> SSQIRQNYSTEVEAAVNRLVNLYLRASYTYLSLGFYFDRDDVALEGVCHFFCELACEKCEGACRLLKMQNQRGGRALFQDLQKP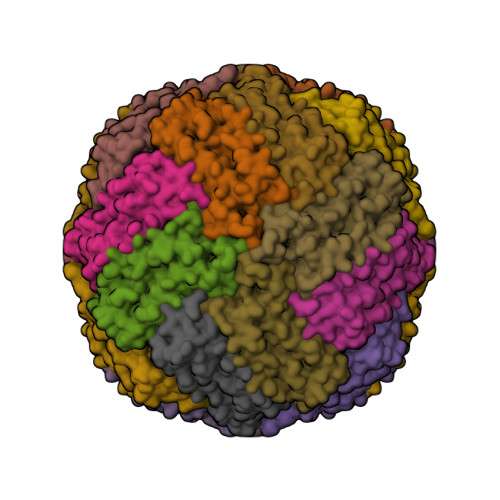SQDEWGTTLDAMKAAIVLEKSLNQALLDLHALGSAQADPHLCDFLESHFLDEEVKLIKKMGDHLTNIQRLVGSQAGLGEYLFERLTLKHD> LGSSNDNIELVDFQNIMFYGDAEVGDNQQPFTFILDTGSANLWVPSVKCTTAGCLTKHLYDSSKSRTYEKDGTKVEMNYVSGTVSGFFSKDLVTVGNLSLPYKFIEVIDTNGFEPTYTASTFDGILGLGWKDLSIGSVDPIVVELKNQNKIENALFTFYLPVHDKHTGFLTIGGIEER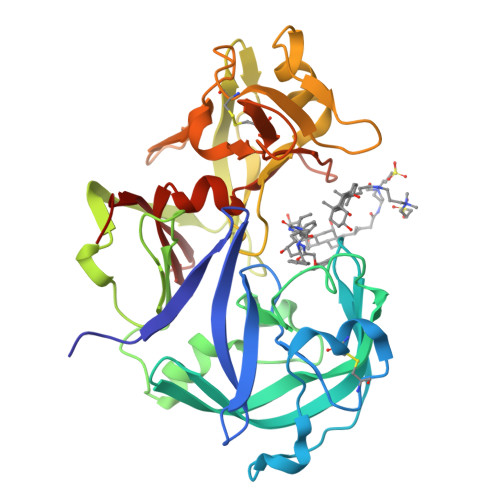FYEGPLTYEKLNHDLYWQITLDAHVGNIMLEKANCIVDSGTSAITVPTDFLNKMLQNLDVIKVPFLPFYVTLCNNSKLPTFEFTSENGKYTLEPEYYLQHIEDVGPGLCMLNIIGLDFPVPTFILGDPFMRKYFTVFDYDNQSVGIALAKKNL>HMPNYKLTYFNMRGRAEIIRYIFAYLDIQYEDHRIEQADWPEIKSTLPFGKIPILEVDGLT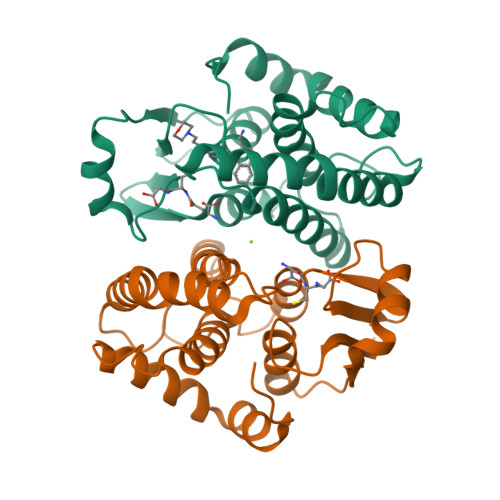LHQSLAIARYLTKNTDLAGNTEMEQCHVDAIVDTLDDFMSCFPWAEKKQDVKEQMFNELLTYNAPHLMQDLDTYLGGREWLIGNSVTWADFYWEICSTTLLVFKPDLLDNHPRLVTLRKKVQAIPAVANWIKRRPQTKL[2x]>[4x]GPGSMKDDHKAQHRFAGLATRAIHSGYRPDPATGAVNAPIYASSTFAQDGVGGLRGGYEYARTGNPTRTALEAALAAVEDAAFGRAFSSGMAAADCALRAMLRPGDHVVIPDDAYGGTFRLIDKVFTGWNVEYTPVALADLDAVRAAIRPTTRLIWVETPTNPLLSIADIAGIAQLGADSSAKVLVDNTFASPALQQPLS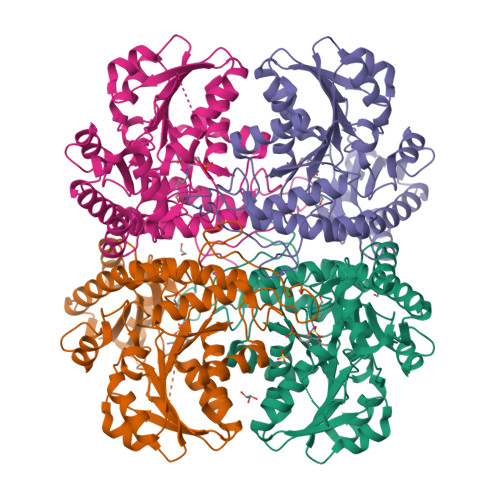LGADVVLHSTTKYIGGHSDVVGGALVTNDEELDQSFAFLQNGAGAVPGPFDAYLTMRGLKTLVLRMQRHSENAAAVAEFLAEHPAISTVLYPGLPSHPGHAVAARQMRGFGGMVSVRMRAGRTAAEQLCAKTNIFILAESLGSVESLIEHPSAMTHASTAGSQLEVPDDLVRLSVGIEDVADLLDDLKQALG>ADKELKFLVVDDFSTMRRIVRNLLKELGFNNVEEAEDGVDALNKLQAGGFGFIISDWNMPNMDGLELLKTIRADSAMSALPVLMVTAEAKKENIIAAAQAGASGYVVKPFTAATLEEKLNKIFEKLGM[4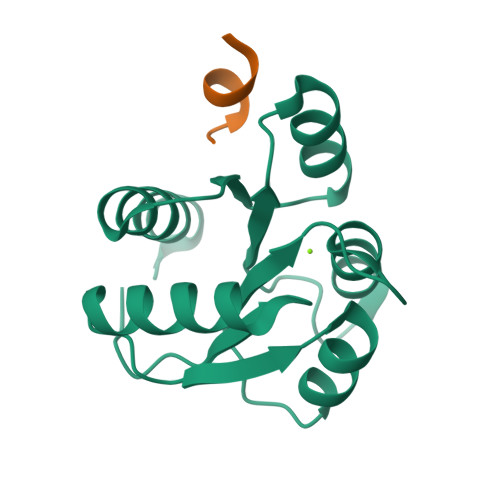x];>[2x]ASQDQVDDLLDSLGF> MQNIVSSKSEQATVIGLVGFYFKDSTFKELMFIQVGEKSNLMNKARINTDAQQIQSIRWMGNLKSPQTGEYRLSTSSDENVILQINGETVINQASIQKNLKLEANQVYEIKIEYRNTSNTLPDLQLFWSMNNAQKEQIPEKYILSPNFSEKANSLAEKETQSFFPNYNLFDRQQENGEKQSMSTPVDTDNDCIPDEWEEKGYTFRNQQIVPWNDAYSAEGYKKYVSNPYHARTVKDPYTDFEKVTGHMPAATKYEARDPLVAAYPSVGVGMEKLHFSKNDTVTEGNADTKSKTTTKTDTTTNTVEIGGSLGFSDKGFSFSISPKYTHSWSSSTSVADTDSTTWSSQIGINTAERAYLNANVRYYNGGTAPIYDLKPTTNFVFQNSGDSITTITAGPNQIGNSLGAGDTYPQKGQAPISLDKANEAGTVKIAINAEQLDKIQAGTEILNIETTQNRGQYGILDEKGQVIPGGEWDPIRTNIDAVSGSLTLNLGTGKDSLERRVAAKNMNDPEDKTPEITIKEAIKKAFNAYYYDGRLYYTDQGEKDIFIDEPSINLITDENTKKEIERQLNQMPGKTVYDVKWKRGMKITLHVPIKYYDFETSENLWYYTYQESGGYTGKKRGRIGTDGHGTAMSNPQLKPYTSYTVRAYVRTASTTGSNEVVFYADNSSGNGQGAKVSGKVTGGKWKIAEFSFNTFNNPEYFKIIGLKNNGNANLHFDDVSVIEWKTNENLQKKHIFEKWSFGSNDEMVIGATFTRVPSSKIRYQWKINGRLGSIIPAPPLDANGKRTVTYGSITAITPMELYAVDEK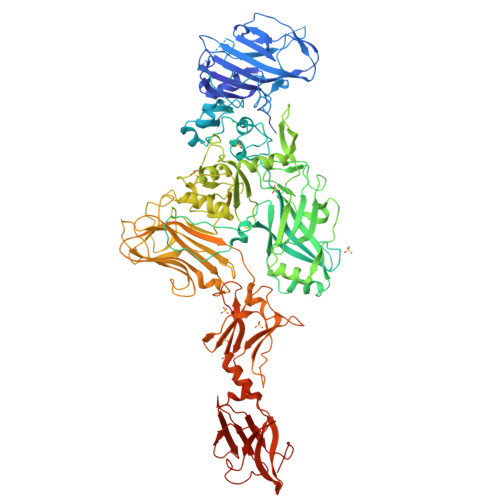NDNLKVKVAELGESEIEKVMIDAHKFSGWWYLSENPNLYSGLSLYKLPDIFYNNVSSYKIRVNGKKVQTVSKPSPFLFQITFNLKNPNGGTYPTKDASVELWATVGGKDLKVLHKWIQKSDVMYSQTNN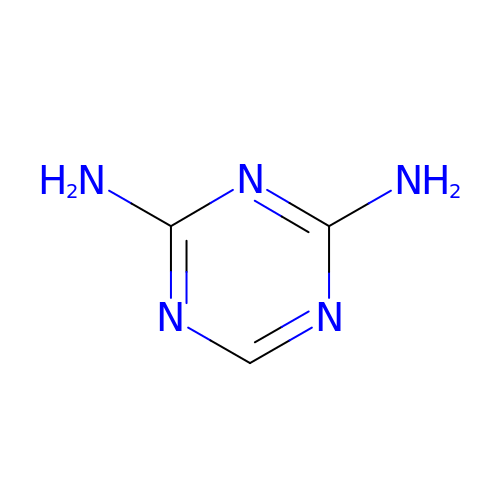1,3,5-TRIAZINE-2,4-DIAMINE | C3 H5 N5 | VZXTWGWHSMCWGA-UHFFFAOYSA-N> MEAGITGTWYNQLGSTFIVTAGADGALTGTYESAVGNAESRY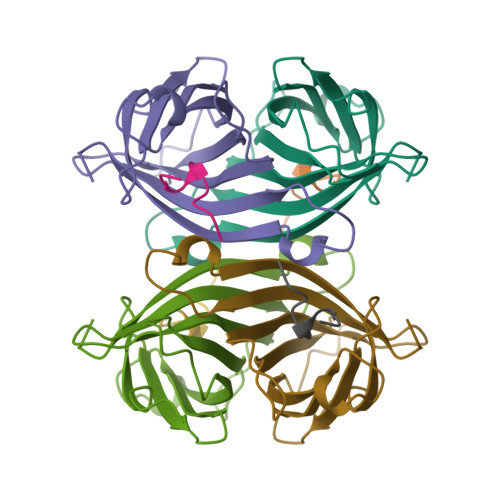VLTGRYDSAPATDGSGTALGWTVAWKNNYRNAHSATTWSGQYVGGAEARINTQWLLTSGTTEANAWKSTLVGHDTFTKVKPSAAS;> AWRHPQFGG>MHHHHHHHKPEDFRASTQRPFTGEEYLKSLQDGREIYIYGERVKDVTTHPAFRNAAASVAQLYDALHKPEMQDSLCWNTDTGSGGYTHKFFRVAKSADDLRQQRDAIAEWSRLSYGWMGRTPDYKAAFGCALGANPGFYGQFEQNARNWYTRIQETGLYFNHAIVNPPIDRHLPTDKVKDVYIKLEKETDAGIIVSGAKVVATNSALTHYNMIGSGSDLGSGSDPDFALMFVAPMDADGVKLISRASYEMVAGATGSPYDYPLSSRFDENDAILVMDNVLIPWENVLIYRDFDRCRRWTMEGGFARMYPLQACVRLAVKLDFITALLKKSLECTGTLEFRGVQADLGEVVAWRNTFWALSDSMCSEATPWVNGAYLPDHAALQTYRVLAPMAYAKIKNIIERNVTSGLIYLPSSARDLNNPQIDQYLAKYVRGSNGMDHVQRIKILKLMWDAIGSEFGGRHELYEINYSGSQDEIRLQCLRQAQNSGNMDKMMAMVDRCLSEYDQDGWTVPHLHNNDDINMLDKLLK[2x]

As an FAD-dependent hydroxylase, 4-hydroxyphenylacetate 3-hydroxylase (HpaB) is able to ortho-hydroxylate phenylpropanoids in a molecular chaperon-independent manner and has broad substrate specificity and high catalytic activity. Among them, the HpaBC complex from E. coli (EcHpaBC) has outstanding activities and a broad substrate spectrum. More interestingly, we found that EcHpaB is also capable of hydroxylating a series of phenylpropanoids to generate a wide range of natural products. The highest titers were reported at 62.7 mg/L and 34.7 mg/L in whole-cell catalysis studies, respectively. These results indicate that EcHpaB has a broad substrate spectrum for the hydroxylation of a variety of phenolic compounds.

In order to further test our hypothesis, mutant XS6 was designed and generated by employing a loop containing residues mainly Gly, Ser, and Asp, which are usually not involved in secondary structure formation. Swiss-model suggested that the β32-β33 loop of XS6 was a random coil. The results of in vitro enzyme assays revealed that XS6 had the almost same specificity constant values (kcat/Km) towards p-coumaric acid and umbelliferone as wild type EcHpaB and had even higher specificity constant values towards larger substrates such as resveratrol and naringenin compared with wild type EcHpaB. The Km values towards p-coumaric acid, umbelliferone, resveratrol and naringenin decreased from 137.6 μM, 217.0 μM, 174.3 μM and 349.8 μM to 132.1 μM, 176.9 μM, 144.0 μM and 191.6 μM, respectively, which indicated XS6 has improved affinity towards all the tested substrates, especially, the largest one, naringenin. To further examine this, we determined the crystal structure of mutant XS6. Compared with wild type EcHpaB, the electron density of residues 208–216 in the loop connecting strands β32-β33 was missing in mutant XS6 (indicated by the dashed line), verifying that the loop in XS6 is highly flexible. The sequence and structural analyses indicated the increased activities of XS6 towards larger substrates are most likely caused by increased loop flexibility that is beneficial to substrate entrance and binding.> MEAPPVTMMPVTGGTINMMEYLLQGSVLDHSLESLIHRLRGLCDNMEPETFLDHEMVFLLKGQQASPFVLRARRSMDRAGAPWHLRYLGQPEMGDKNRHALVRNCVDIATSENLTDFLMEMGFRMDHEFVAKGH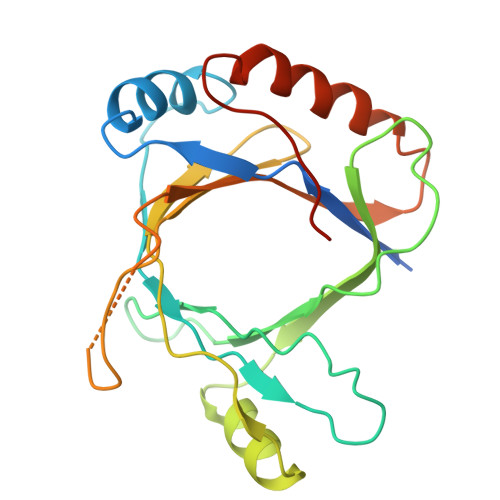LFRKGIMKVVVYKIFRILVPGNTDSTEALSLSYLVELSVVAPAGQDMVSDDMRNFAEQLKPLVHLEKIDPKRLM>[6x]MIANENIQDKALE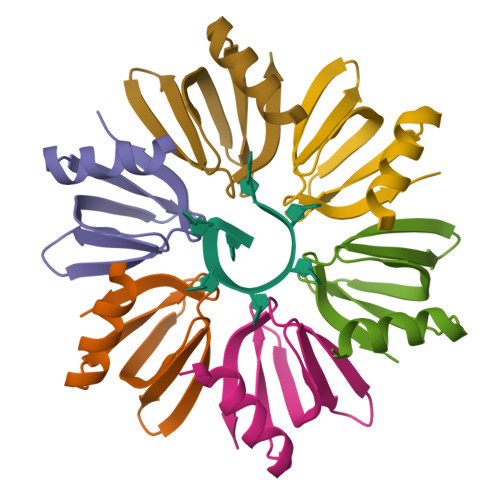NFKANQTEVTVFFLNGFQMKGVIEEYDKYVVSLNSQGKQHLIYKHAISTYTVETEGQASTESEE> MASQPNSSAKKKEEKGKNIQVVVRCRPFNLAERKASAHSIVECDPVRKEVSVRT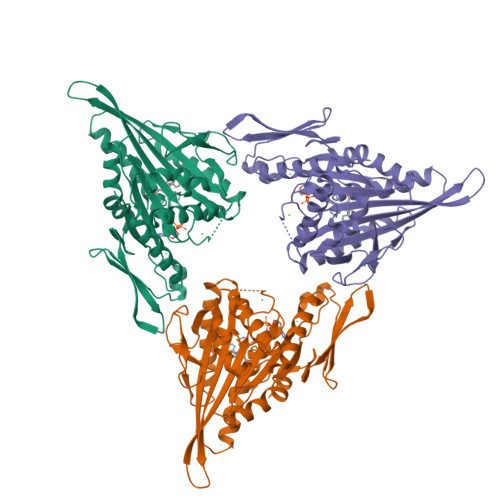GGLADKSSRKTYTFDMVFGASTKQIDVYRSVVCPILDEVIMGYNCTIFAYGQTGTGKTFTMEGERSPNEEYTWEEDPLAGIIPRTLHQIFEKLTDNGTEFSVKVSLLEIYNEELFDLLNPSSDVSERLQMFDDPRNKRGVIIKGLEEITVHNKDEVYQILEKGAAKRTTAATLMNAYSSRSHSVFSVTIHMKETTIDGEELVKIGKLNLVDLAGSENIGRSGAVDKRAREAGNINQSLLTLGRVITALVERTPHVPYRESKLTRILQDSLGGRTRTSIIATISPASLNLEETLSTLEYAHRAKNILNKPEVNQK> MDKDEAWKQVEQ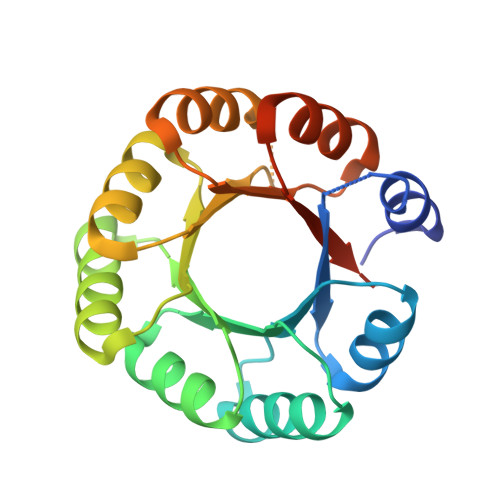LRREGATQIAYRSDDWRDLKEAWKKGADILIVDATDKDEAWKQVEQLRREGATQIAYRSDDWRDLKEAWKKGADILIVDATDKDEAWKQVEQLRREGATQIAYRSDDWRDLKEAWKKGADILIVDATDKDEAWKQVEQLRREGATQIAYRSDDWRDLKEAWKKGADILIVDATGLEHHHHHH> MQSARAKKSNEF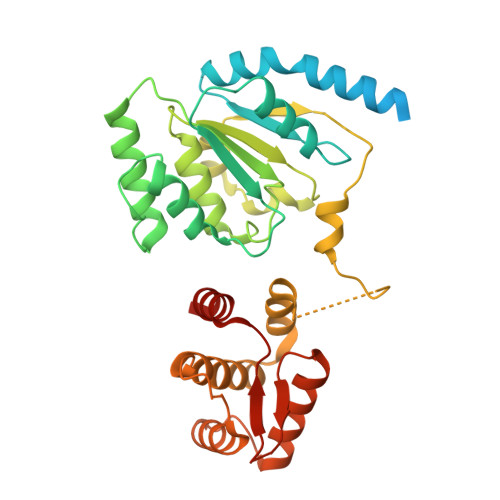VPESDGYFHSHASSKILTSDHTLDRLKNPRLAADRVFSLLSEIKTSAEHEGSINAIMEEYRSYFPKWMCILNEGFNILLYGLGSKHQLLQSFHREVLHKQTVLVVNGFFPSLTIKDMLDSITSDILDAGISPANPHEAVDMIEEEFALIPETHLFLIVHNLDGAMLRNVKAQAILSRLARIPNIHLLASIDHINTPLLWDQGKLCSFNFSWWDCTTMLPYTNETAFENSLLVQNSGELALSSMRSVFSSLTTNSRGIYMLIVKYQLKNKGNATYQGMPFRDLYSSCREAFLVSSDLALRAQLTEFLDHKLVKSKRSVDGSEQLTIPIDGALLQQFLEEQEKK> ATSSPNVQVYTYKLIKEGESNVLLCHAKDFSPPNIKLELLENGRIIPNTTQSDLSFES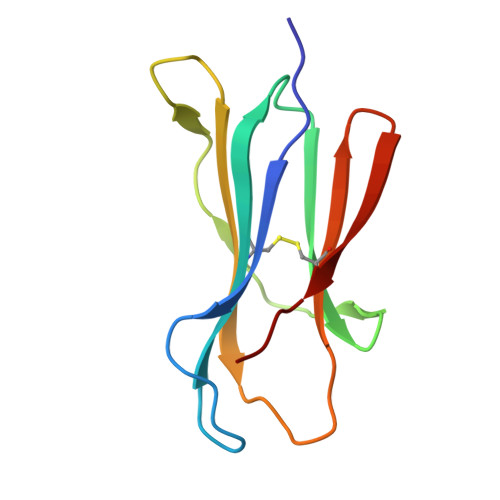DWSFKLTRYVEFTPQSGYKYSCMVTHNGDSKEIQLDRY> MLEQPYLDLAKKVLDEGHFKPDITHTGTYSIFGHQMRFDLSKGFPLLTTKKVPFGLIKSELLWFLHGDTNIRFLLQHRNHIWDEWAFEKWVK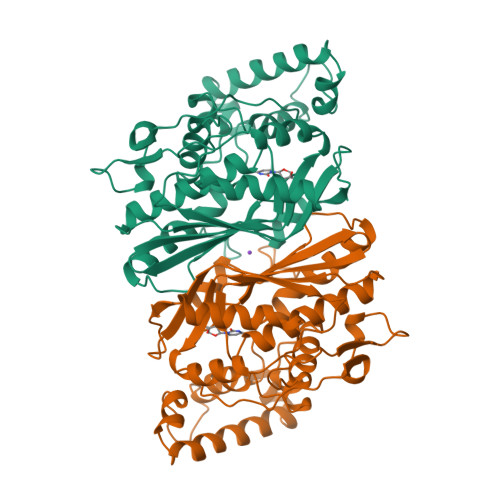SDEYHGPDMTDFGHRSQKDPEFAAVYHEEMAKFDDRVLHDDAFAAKYGDLGLVYGSQWRAWHTSKGDTIDQLGDVIEQIKTHPYSRRLIVSAWNPEDVPTMALPPCHTLYQFYVNDGKLSLQLYQRSADIFLGVPFNIASYALLTHLVAHECGLEVGEFIHTFGDAHLYVNHLDQIKEQLSRTPRPAPTLQLNPDKHDIFDFDMKDIKLLNYDPYPAIKAPVAV>MNNTIETILNHRSIRSFTDQLLTAEEIDTLVKSAQAASTSSYVQAYSIIGVSDPEKKRELSVLAGNQPYVEKNGHFFVFCADLYRHQQLAEEKGEHISELLENTEMFMVSLIDAALAAQNMSIAAESMGLGICYIGGIRNELDKVTEVLQTPDHVLPLFGLAVGHPANLSGKKPRLPKQAVYHENTYNVNTDDFRHTMNTYDKTISDYYRERTNGKREETWSDQILNFMKQKPRTYLNDYVKEKGFN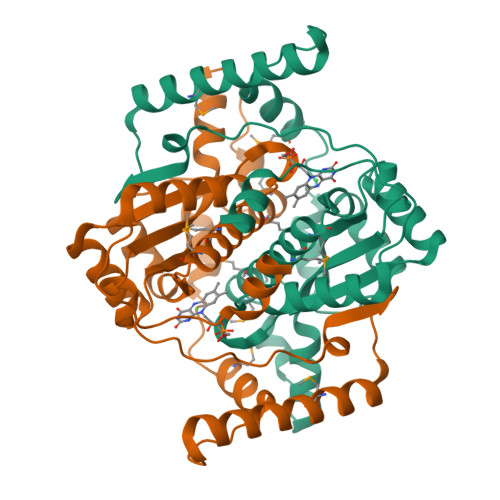KN[4x]> MEQLTKCEVFQKLKDLKDYGGVSLPEWVCIAFHTSGYDTQAIVQNNDSTEYGLFQINNKIWCKDDQNPHSRNICNISCDKFLDDDLTDDIVCAKKILDKVGINYWLAHKALCSEKL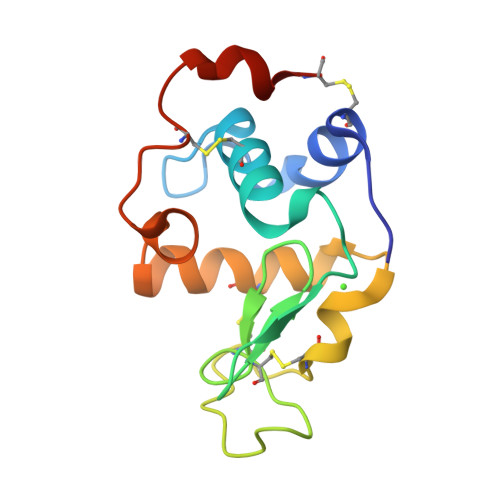DQWLCEKL>HHPCCSNPCQNRGECMSTGFDQYKCDCTRTGFYGENCTTPEFLTRIKLLLAPTPQTVHYILTHFKGVWNIVNNVPFLRSLIMKYVLTSRPYLIDSPPTYNVHYGYKSWEAFSNLSYYTRALPPVADDCPTPMGVKGNKELPDSKEVLEKVLLRREFIPDPQGSNMMFAFFAQHFTHQFFKTDHKRGPGFTRGLGHGVDLNHIYGETLDRQHKLRLFKDGKLKYQVIGGEVYPPTVKDTQVEMIYPPHIPENLQFAVGQEVFGLVPGLMMYATIWLREHNRVCDILKQEHPEWGDEQLFQTSRLILIGETIKIVIEDYVQHLSGYHFKLKFDPELLFNQQFQYQNRIASEFNTLYHWHPLLPDTFNIEDQEYSFKQFLYNNSILLEHGLTQFVESFTRQIAGRVAGGRNVPIAVQAVAKASIDQSREMKYQSL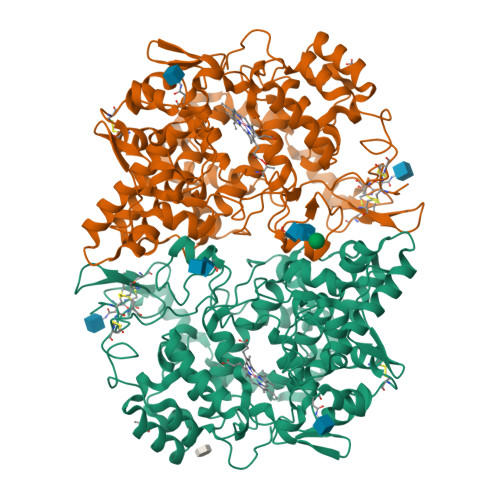NEYRKRFSLKPYTSFEELTGEKEMAAELKALYSDIDVMELYPALLVEKPRPDAIFGETMVELGAPFSLKGLMGNPICSPQYWKPSTFGGEVGFKIINTASIQSLICNNVKGCPFTSFNV[2x]> ALKPCEFPQFKYGRLYYEESLRPNFPVSIGNKYSYKCDNGFSPPSGYSWDYLRCTAQGWEPEVPCVRKCVFHYVENGDSAYWEKVYVQGQSLKVQCYNGYSLQNGQDTMTCTENGWSPPPKCIR

Factor H binding protein (fHbp) is a 27 kDa surface lipoprotein consisting of two β-barrels that promotes resistance against complement mediated lysis and is a key meningococcal antigen that elicits SBAs. We have shown previously that fH CCP 6 and 7 (fH67) are necessary for high affinity interactions with V1 fHbp, and that these two CCPs are sufficient to inhibit binding of full length fH to fHbp. Here we characterised members of the three variant families by identifying amino acids that are critical for fH binding and through structural analysis, to inform future vaccine design and to understand the basis of the interaction of fHbp with fH. Here we show that even though V1, 2 and V3 fHbps exhibit remarkably conserved atomic structures, differences in key amino acids necessary for interactions with fH are only revealed by functional studies.

As fHbp binds human (hfH) but not murine fH (mfH), novel models are required to assess the efficacy of fHbp-based vaccines. Therefore to develop a physiologically relevant model to test non-functional fHbp vaccines, we sought to define the basis of the binding of fHbp to hfH but not mfH. Alignment of the amino acid sequences of hfH and mfH revealed multiple residues located at the site of interaction with fHbp that differ between the two species. Therefore, we next humanised 13 residues in mfH that span the region corresponding to the interaction site of hfH with fHbp. However this extensive replacement of residues was not sufficient to enable mfH to bind fHbp at appreciable levels as demonstrated by far Western analysis; PPX, the meningococcal exo-polyphosphatase was used as a control on blots. The overall CCP folds are conserved despite many sequence differences between the two species throughout the two structures, including the surface where hfH interacts with fHbp. Additionally the arrangement of CCPs 6 and 7 in mfH with respect to each other is distinct from hfH, distorting the entire shape of the potential interface with fHbp. We also demonstrate that impaired binding of the murine fH to fHbp is not solely due to amino acid differences at the binding site; structural analyses revealed a different orientation of CCPs 6 with 7 in the human and murine molecules that would sterically inhibit interactions with mfH. Initial efforts to achieve this by introducing multiple amino acid changes in mfH proved unsuccessful, most likely due to the orientation of CCP 6 with 7 in mfH which would sterically inhibit interactions with fHbp. The chimeric fH consists of mfH CCPs 1–5 and 9–20 (enabling interaction with murine C3b and other complement components), flanking hfH CCPs 6–8 (allowing binding to fHbp).> KELVLALYDYQEKGDSEVTMKKGDILTLLNSTN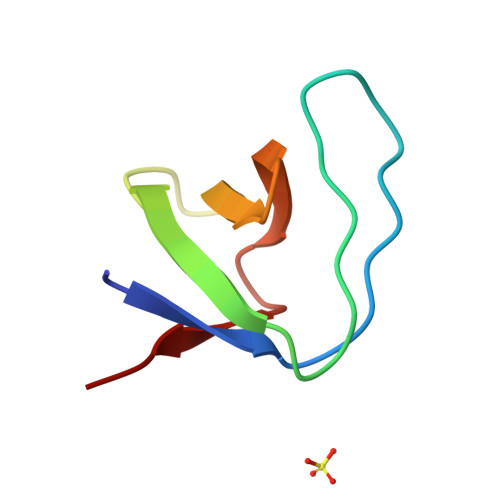KDWWKVEVNDRQGFVPAAYVKKLD> SENLYFQGSGSLFFSFFKTLVDQEVVVELKNDIEIKGTLQSVDQFLNLKLDNISCTDEKK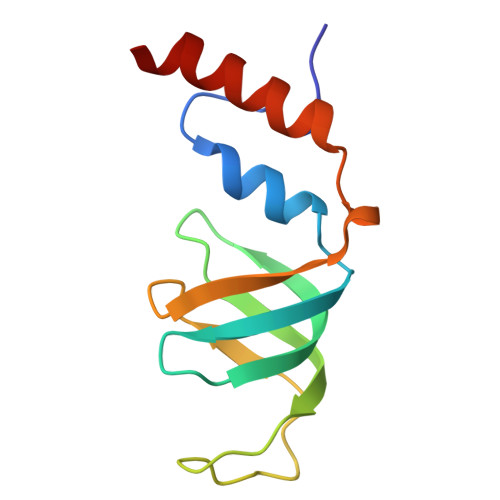YPHLGSVRNIFIRGSTVRYVYLNKNMVDTNLLQDATRREVMTERK(1R,2R)-2-[(2S,6E,8R,9S,11R,13S,15S,16S)-7-cyano-8,16-dihydroxy-9,11,13,15-tetramethyl-18-oxooxacyclooctadec-6-en-2-yl]cyclobutanecarboxylic 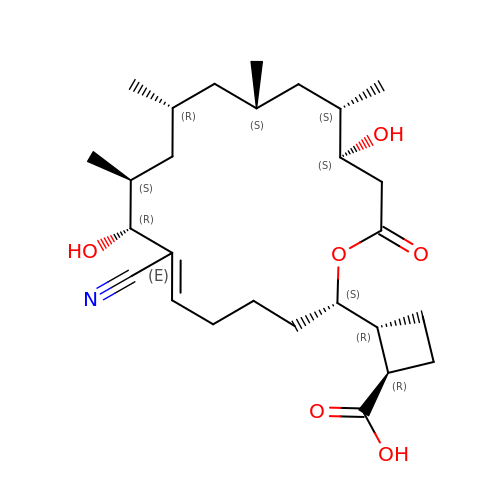acid | C27 H43 N O6 | KHMHNBNVTBTHJD-IIZLMIOOSA-N5-(aminomethyl)pyridin-2-amine | C6 H9 N3 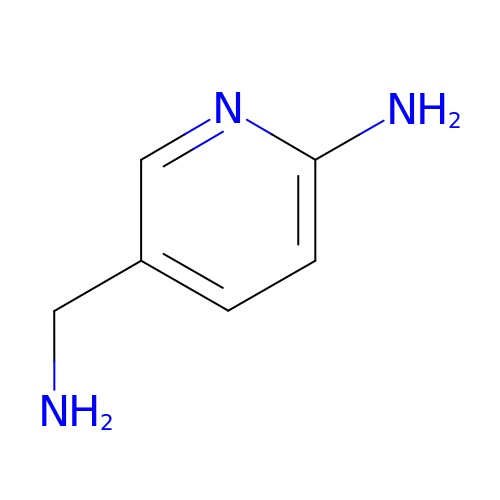| PHBVTMQLXNCAQO-UHFFFAOYSA-N> MSMLKREDWYDLTRTTNWTPKYVTENELFPEEMSGARGISMEAWEKYDEPYKITYPEYVSIQREKDSGAYSIKAALERDGFVDRADPGWVSTMQLHFGAIALEEYAASTAEARMARFAKAPGNRNMATFGMMDENRHGQIQLYFPYANVKRSRKWDWAHKAIHTNEWAAIAARSFFDDMMMTRDSVAVSIMLTFAFETGFCNMQFLGLAADAAEAGDHTFASLISSIQTDESRHAQQGGPSLKILVENGKKDEAQQMVDVAIWRSWKLFSVLTGPIMDYYTPLESRNQSFKEFMLEWIVAQFERQLLDLGLDKPWYWDQFMQDLDETHHGMHLGVWYWRPTVWWDPAAGVSPEEREWLEEKYPGWNDTWGQCWDVITDNLVNGKPELTVPETLPTICNMCNLPIAHTPGNKWNVKDYQLEYEGRLYHFGSEADRWCFQIDPERYENHTNLVDRFLKGEIQPADLAGALMYMSLEPGVMGDDAHDYEWVKAYQKKTNAA;> MSEQQPEALKPLKTWSHLAGNRRRPSEYEVVSTNLHYFTDNPERPWELDSNLPMQTWYKKYCFDSPLKHDDWN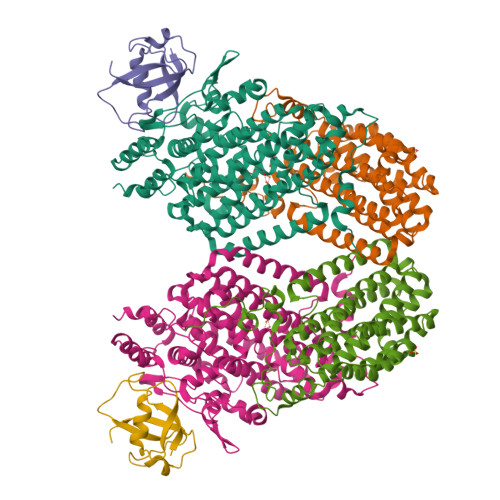AFRDPDQLVYRTYNLLQDGQESYVQGLFDQLNDRGHDQMLTREWVETLARFYTPARYLFHALQMGSVYIHQIAPASTITNCATYETADHLRWLTHTAYRTRELANCYPDVGFGKRERDVWENDPAWQGFRELIEKALIAWDWGEAFTAINLVTKPAVEEALLQQLGSLAQSEGDTLLGLLAQAQKRDAERHRRWSSALVKMALEKEGNREVLQKWVAKWEPLADKAIEAYCSALPDGENAIVEAKSASRYVRQMMGL;> MATFPIMSNFERDFVIQLVPVDTEDTMDQVAEKCAYHSINRRVHPQPEKILRVRRHEDGTLFPRGMIVSDAGLRPTETLDIIFMDN>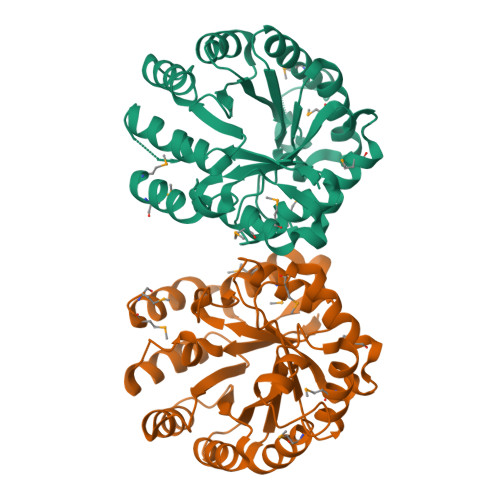MSLGKRIFVFDTTLRDGEQVPGCQLNTEEKIIVAKALDELGVDVIEAGFPVSSPGDFNSVVEITKAVTRPTICALTRAKEADINIAGEALRFAKRSRIHTGIGSSDIHIEHKLRSTRENILEMAVAAVKQAKKVVHEVEFFCEDAGRADQAFLARMVEAVIEAGADVVNIPDTTGYMLPWQYGERIKYLMDNVSNIDKAILSAHCHNDLGLATANSLAALQNGARQVECTINGIGERAGNTALEEVVMAMECHKETLGLETGINHKKLVPISHLVSTLMRMQVQSNKAIVGRNAFAHSSGIHQDGFLKHRETYEIIDEGHHHHHH[2x]>FEGDLKWHHHNITYWIQNYSEDLPRAVIDDAFARAFALWSAVTPLTFTRVYSRDA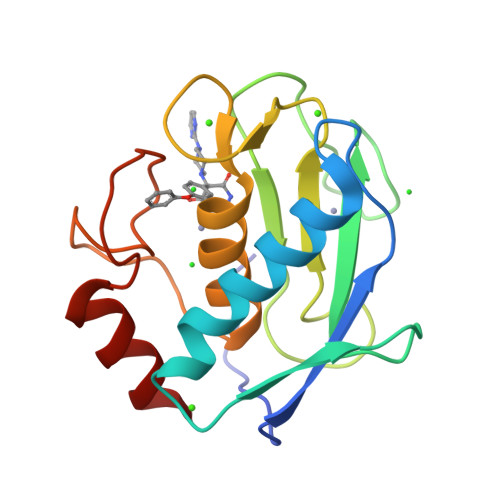DIVIQFGVAEHGDGYPFDGKDGLLAHAFPPGPGIQGDAHFDDDELWSLGKGQGYSLFLVAAHQFGHALGLDHSSVPEALMYPMYRFTEGPPLHKDDVNGIRHLY[2x]9H-PURINE-2,6-DIAMINE | C5 H6 N6 | 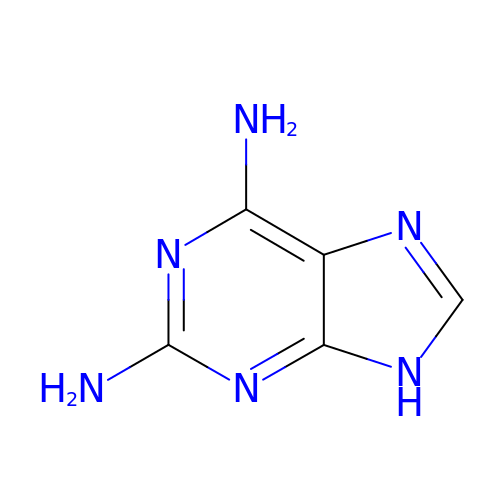MSSXOMSJDRHRMC-UHFFFAOYSA-N>[3x]MEPHVLGAGLYWLLLPCTLLAASLLRFNALSLVYLLFLLLLPWLPGPSRHSIPGHTGRLLRALLCLSLLFLVAHLAFQICLHTVPHLDQFLGQNGSLWVKVSQHIGVTRLDLKDIFNTTRLVAPDLGVLLASSLCLGLCGRLTRKAGQSRRTQELQDDDDDDDDDDEDIDAAPAVGLKGAPALATKRRLWLASRFRVTAHWLLMTSGRTLVIVLLALAGIAHPSAFSSIYLVVFLAICTWWSCHFPLSPLGFNTLCVMVSCFGAGHLICLYCYQTPFIQDMLPPGNIWARLFGLKNFVDLPNYSSPNALVLNTKHAWPIYVSPGILLLLYYTATSLLKLHKSCPSELRKETPREDEEHELELDHLEPEPQARDATQGEMPMTTEPDLDNCTVHVLTSQSPVRQRPVRPRLAELKEMSPLHGLGHLIMDQSYVCALIAMMVWSIMYHSWLTFVLLLWACLIWTVRSRHQLAMLCSPCILLYGLTLCCLRYVWAMELPELPTTLGPVSLHQLGLEHTRYPCLDLGAMLLYLLTFWLLLRQFVKEKLLKKQKVPAALLEVTVADTEPTQTQTLLRSLGELVTGIYVKYWIYVCAGMFIVVSFAGRLVVYKIVYMFLFLLCLTLFQVYYTLWRKLLRVFWWLVVAYTMLVLIAVYTFQFQDFPTYWRNLTGFTDEQLGDLGLEQFSVSELFSSILIPGFFLLACILQLHYFHRPFMQLTDLEHVPPPGTRHPRWAHRQDAVSEAPLLEHQEEEEVFREDGQSMDGPHQATQVPEGTASKWGLVADRLLDLAASFSAVLTRIQVFVRRLLELHVFKLVALYTVWVALKEVSVMNLLLVVLWAFALPYPRFRPMASCLSTVWTCIIIVCKMLYQLKIVNPHEYSSNCTEPFPNNTNLQPLEINQSLLYRGPVDPANWFGVRKGYPNLGYIQNHLQILLLLVFEAVVYRRQEHYRRQHQQAPLPAQAVCADGTRQRLDQDLLSCLKYFINFFFYKFGLEICFLMAVNVIGQRMNFMVILHGCWLVAILTRRRREAIARLWPNYCLFLTLFLLYQYLLCLGMPPALCIDYPWRWSKAIPMNSALIKWLYLPDFFRAPNSTNLISDFLLLLCASQQWQVFSAERTEEWQRMAGINTDHLEPLRGEPNPIPNFIHCRSYLDMLKVAVFRYLFWLVLVVVFVAGATRISIFGLGYLLACFYLLLFGTTLLQKDTRAQLVLWDCLILYNVTVIISKNMLSLLSCVFVEQMQSNFCWVIQLFSLVCTVKGYYDPKEMMTRDRDCLLPVEEAGIIWDSICF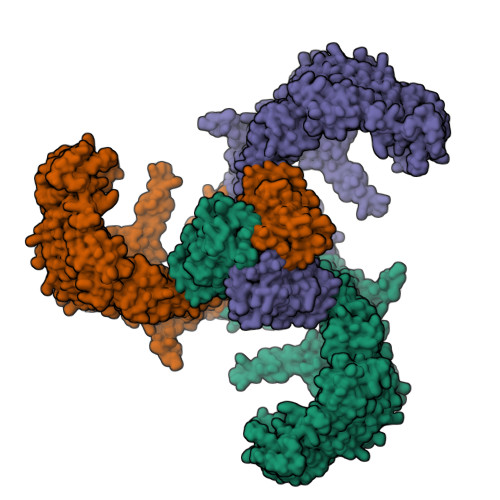FFLLLQRRIFLSHYFLHVSADLKATALQASRGFALYNAANLKSINFHRQIEEKSLAQLKRQMKRIRAKQEKYRQSQASRGQLQSKDPQDPSQEPGPDSPGGSSPPRRQWWRPWLDHATVIHSGDYFLFESDSEEEEEALPEDPRPAAQSAFQMAYQAWVTNAQTVLRQRRERARQERAEQLASGGDLNPDVEPVDVPEDEMAGRSHMMQRVLSTMQFLWVLGQATVDGLTRWLRAFTKHHRTMSDVLCAERYLLTQELLRVGEVRRGVLDQLYVGEDEATLSGPVETRDGPSTASSGLGAEEPLSSMTDDTSSPLSTGYNTRSGSEEIVTDAGDLQAGTSLHGSQELLANARTRMRTASELLLDRRLHIPELEEAERFEAQQGRTLRLLRAGYQCVAAHSELLCYFIIILNHMVTASAASLVLPVLVFLWAMLTIPRPSKRFWMTAIVFTEVMVVTKYLFQFGFFPWNSYVVLRRYENKPYFPPRILGLEKTDSYIKYDLVQLMALFFHRSQLLCYGLWDHEEDRYPKDHCRSSVKDREAKEEPEAKLESQSETGTGHPKEPVLAGTPRDHIQGKGSIRSKDVIQDPPEDLKPRHTRHISIRFRRRKETPGPKGTAVMETEHEEGEGKETTERKRPRHTQEKSKFRERMKAAGRRLQSFCVSLAQSFYQPLQRFFHDILHTKYRAATDVYALMFLADIVDIIIIIFGFWAFGKHSAATDIASSLSDDQVPQAFLFMLLVQFGTMVIDRALYLRKTVLGKLAFQVVLVVAIHIWMFFILPAVTERMFSQNAVAQLWYFVKCIYFALSAYQIRCGYPTRILGNFLTKKYNHLNLFLFQGFRLVPFLVELRAVMDWVWTDTTLSLSNWMCVEDIYANIFIIKCSRETEKKYPQPKGQKKKKIVKYGMGGLIILFLIAIIWFPLLFMSLIRSVVGVVNQPIDVTVTLKLGGYEPLFTMSAQQPSIVPFTPQAYEELSQQFDPYPLAMQFISQYSPEDIVTAQIEGSSGALWRISPPSRAQMKQELYNGTADITLRFTWNFQRDLAKGGTVEYTNEKHTLELAPNSTARRQLAQLLEGRPDQSVVIPHLFPKYIRAPNGPEANPVKQLQPDEEEDYLGVRIQLRREQVGTGASGEQAGTKASDFLEWWVIELQDCKADCNLLPMVIFSDKVSPPSLGFLAGYGIVGLYVSIVLVVGKFVRGFFSEISHSIMFEELPCVDRILKLCQDIFLVRETRELELEEELYAKLIFLYRSPETMIKWTRERE>[4x]MRTLKELERELQPRQHLWYFEYYTGNNVGLFMKMNRVIYSGQSDIQRIDIFENPDLGVVFALDGITMTTEKDEFMYHEMLAHVPMFLHPNPKKVLIIGGGDGGTLREVLKHDSVEKAILCEVDGLVIEAARKYLKQTSCGFDDPRAEIVIANGAEYVRKFKNEFDVIIIDSTDPTAGQGGHLFTEEFYQACYDALKEDGVFSAETEDPFYD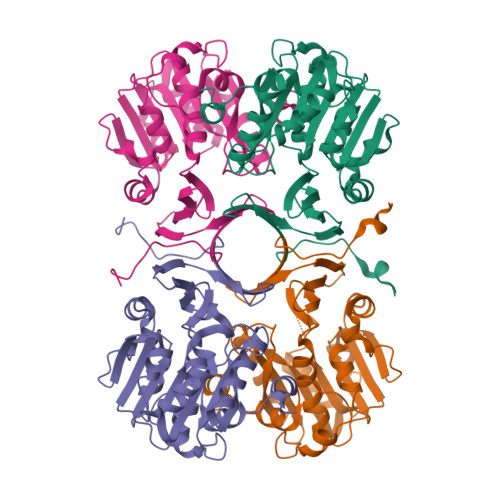IGWFKLAYRRISKVFPITRVYLGFMTTYPSGMWSYTFASKGIDPIKDFDPEKVRKFNKELKYYNEEVHVASFALPNFVKKELGLM> MTVQCKPIPALYTVYVLRSTVRHASLYIGSTPNPPRRLKQHNGLVPGGAARTSRSSLRPWEMVALVSGFPSMVAALKFQWALTNPHLSVHIPSASRLTVATQTKANGRPQRPPRSLASVVANLHLLLRVPSFARWPLRVHFFRRDVFAAWEKWCAAASERLRPSL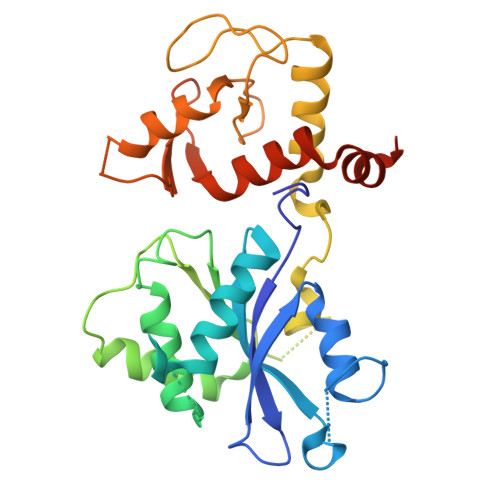AVVTDFEGGSEGLAGAVVGGEEGRERGEGAPCWGIHALPLDYEPIKDYVAKGQEIFEFERQGACVVCREEMASGDGLQALCTNQGCDGVGHLSCWSRHFLKGAEADSILPVQGQCPKCGGEMEWGNMMKELTLRTRGQKEVEKLLKRKRRRATKKTANA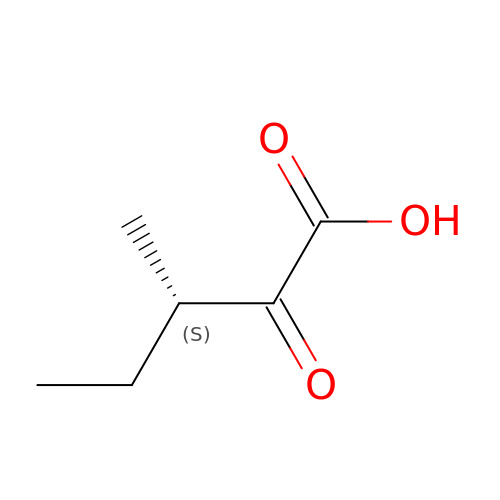(3S)-3-methyl-2-oxopentanoic acid | C6 H10 O3 | JVQYSWDUAOAHFM-BYPYZUCNSA-N4-HYDROXYPHENACYL COENZYME A | C29 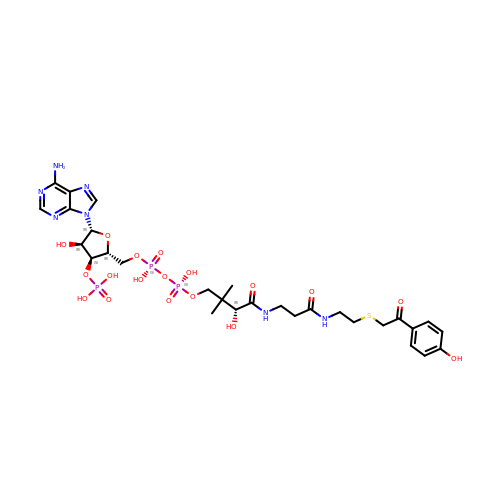H42 N7 O18 P3 S | ZQLMPRRTUJBILA-VXAHOBLNSA-N> MEDENILRNAVNLQVLKFHYPEIESIIDIASHVAVYQFDVGSQKWLKTSIEGTFFLVKDQRARVGYVILNRNSPENLYLFINHPSNVHLVDRYLIHRTENQHVVGLWMFDPNDMSRIFNIVKESLLR;> MSFTNATFSQVLDDLSARFILNLPAEEQSSVERLCFQIEQAHWFYEDFIRAQNDQ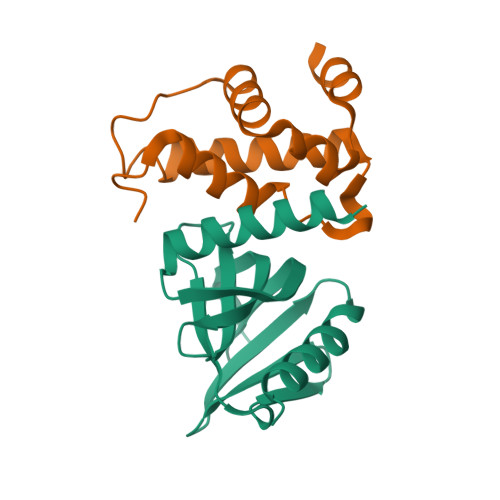LPSLGLRVFSAKLFAHCPLLWKWSKVHEEAFDDFLRYKTR>[2x]MTTKPFFDAARVIAGGKLTQAQVDELNKVVNKLAPGGKTTSDVGVNLISGFEGTRFTAYDDGVGIWTIGTGTTV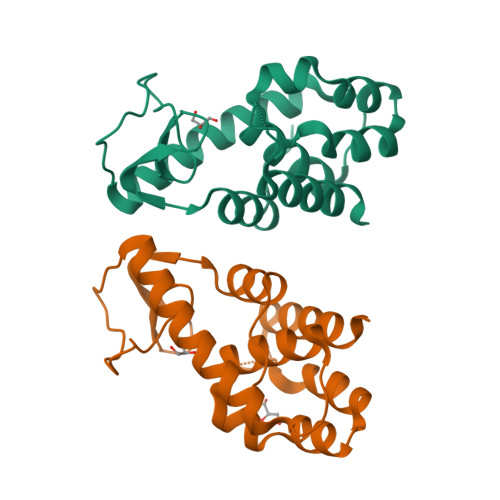YPNGVKVKKGDTCTPEQAKSYFKHDLAKFEKTVNESVTVPLTQNQFDALVSLTYNIGAGALKNSTLLKLLNKGDYKGAADQFLVWNKAGGKVLKGLVRRREAERALFLKK> AAMKISRIAQRLDEAAVSGKATPQLTGDDAVTVREAAEIQRLLIAHRIERGARQVGLKMGFTSRAKMAQMGVSDLIWGRLTSDMWVEEGGEIDLAHYVHPRVEPEICYLLGKRLEGNVTPLEALAAVEAVAPAMEIIDSRYRDFKFSLPDVIADNASSSGFVVGAWHKPETDVSNLGMVMSFDGRAVELGTSAAILGSPIRALVAAARLAAQQG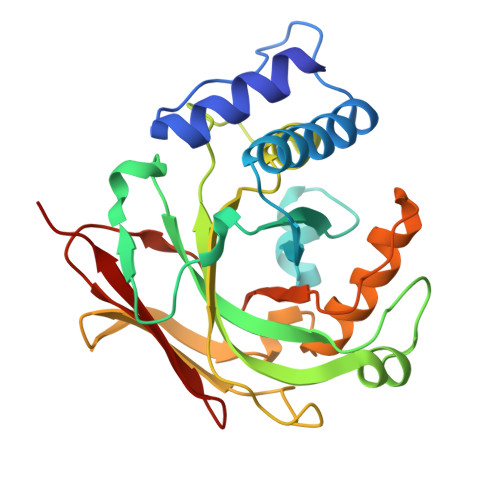EALEAGSLILAGAATAAVALRPGISVRCEVQNLGSLSFSTTGER>[30x]MATPWSGYLDDVSAKFDTGVD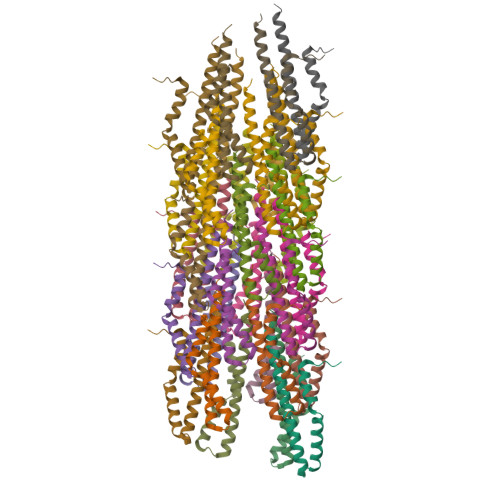NLQTQVTEALDKLAAKPSDPALLAAYQSKLSEYNLYRNAQSNTVKVFKDIDAAIIQNFR> MDTEVSNHNYTQAVAYLNRATSSCVKKCDSLNNNGSL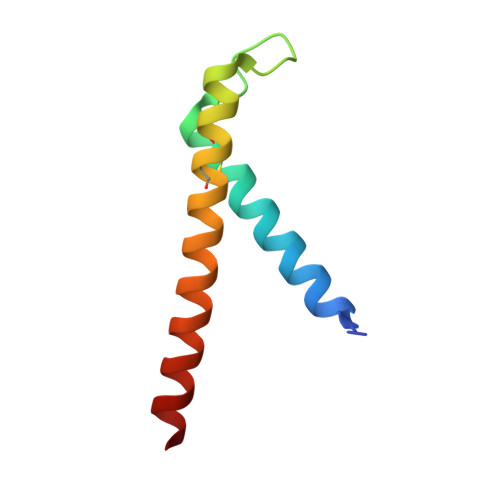SSKQESCLKTCAENHAIATKIHAEYIRKLAESKYL>[4x]MATLFQVSMGSMRHRRNGNFESSRLLYSSMSRSIDVACSDADLANFIQENFKKRECVFFTKDTKSMGNLCKCGYPENQHIEGTQVNTTEKWNYKKHXXXXXXXXXXXXXXXXXXXXXKYIRLSCDTDSETLYDLMTQHWHLKTPNLVISVTGGAKNFALKPRMRKIFSRLIYIAQSKGAWIFTGGTHYGLMKYIGEVVRDNTISRSSEENVVAIGIAAWGMISNRETLIRTADSDGSYLAHYIMDDLKRDPLYCLDNNHTHLLLVDNGTHGHPTIEAKVRTQLEKYISERVIPESNYGGKIPIVCFAQGGGKET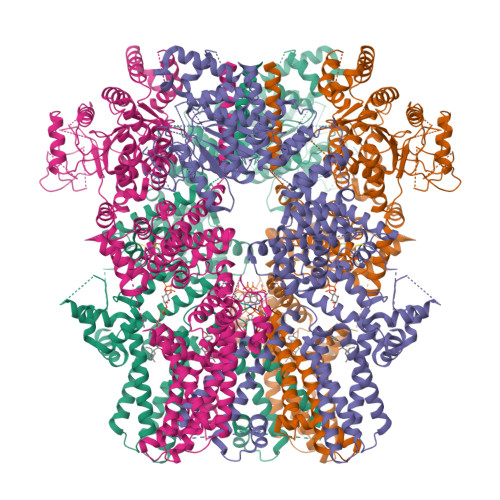LKSINVAIKSKIPCVVVEGSGRIADVIASLVEAEGTLASSCVKESLLRFLPRTISRLSEEETESWIKWIKEVLESPHLLTVIKIEEAGDEIVSNAISFALYKAFSTNEHDRDNWNGQLKLLLEWNQLDLASDEIFTNDRNWESADLQDVMFTALVKDRPKFVRLFLENGLNLRKFLTTEVLRELYTNNFSSLVFKNLQIAKNSYNDALLTFVWKMVEDFRRGAKRDDKNSKDEMEIELSEECPITRHPLQALFIWSVLQNKKELSKVIWEQTRGCTLAALGASKLLKSMAKVKNDINAAGESEELANEYETRAVELFTECYSNDEDLAEQLLTYSCEAWGGSNCLELAVEARDQQFIAQPGVQNFLSKQWYGEISRDTKNWKIILCLFFFPLIGCGFISFRKKPVEKTKKLFLYYVSFFTSPFVVFSWNVIFYIAFLLLFAYVLLMDFQKEPTALEIILYVLVFILLCDEVRQWYMNGSKYFSDLWNVMDTLAIFYFIAGIVFRLHSDESSWYSGRVIFCLDYIVFTLRLIHIFTVSRNLGPKIIMLQRMMIDVFFFLFLFAVWMVAFGVARQGILRKNEHRWEWIFRSVIYEPYLAMFGQYPDDIDGTTYNFDHCTFSGNESKPLCVELDANNQPRFPEWITIPLVCIYMLSTNILLVNLLVAMFGYTVGSVQENNDQVWKFQRFFLVQEYCSRLTIPFPFVIFAYIFMVMRKCFKCCCKKESKEPSVCCSRNEDNEILAWEAVMKENYLVKINTKASDSSEEXXXXXXXXXXXXXXXXXXXXXXXXKIKSNSLEVLFQGPDYKDDDDKAHHHHHHHHHH> GHMVMSTP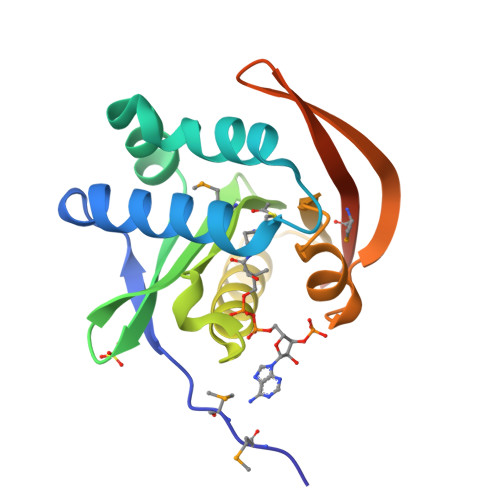ALRPYLPEDAAVTAAIFVASIEQLTADDYSEEQQEAWASAADDEAKFAARLSGQLTLIATLQGVPVGFASLKGPDHIDMLYVHPDYVGRDVGTTLIDALEKLAGARGALILTVDASDNAAEFFAKRGYVAKQRNTVSINGEWLANTTMTKSLADSAAPGASSGS> ADP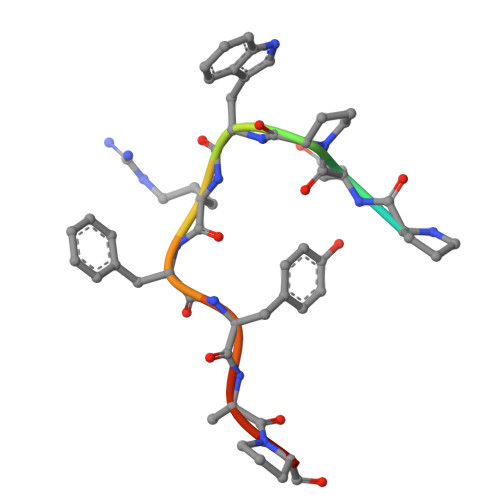QPWRFYAPR> GSGELNVSPFVFRENVMVGEKV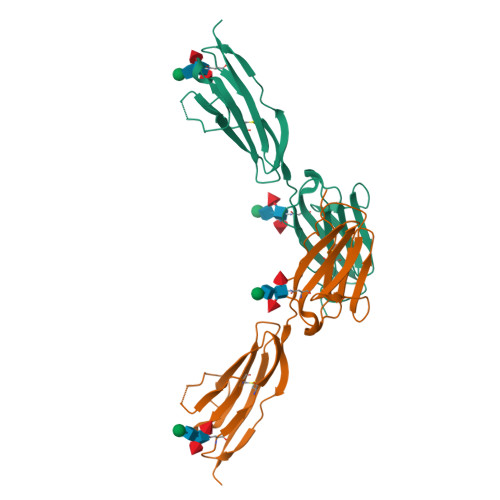TATCTTVTEDAQISFKWFKNGKQINDNEHIKVLYYTDFSLLSINPVKADDSGNYTCVITAKEKSSKFTATLTVKASPEWLIQPENVESVMGSNISLQCSVTGIPTPTINWKKSETSSGTDFKSLSTSSNAIILPGGTLNLLRIIKSDEGLYECQASNGIGNDLRKTVTISVFIP>[2x]VEYRNWSKPQCQITGFAPFSKDNSIRLSAGGDIWVTREPYVSCDPV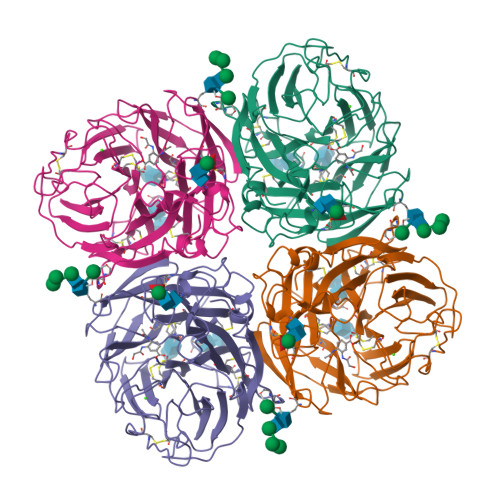KCYQFALGQGTTLDNKHSNDTVHDRIPHRTLLMNELGVPFHLGTRQVCIAWSSSSCHDGKAWLHVCITGDDKNATASFIYDGRLVDSIGSWSQNILRTQESECVCINGTCTVVMTDGSASGRADTRILFIEEGKIVHISPLAGSAQHVEECSCYPRYPGVRCICRDNWKGSNRPVVDINMEDYSIDSSYVCSGLVGDTPRNDDRSSNSNCRDPNNERGTQGVKGWAFDNGNDLWMGRTISKDLRSGYETFKVIGGWSTPNSKSQINRQVIVDSDNRSGYSGIFSVEGKSCINRCFYVELIRGRKQETRVWWTSNSIVVFCGTSGTYGTGSWPDGANINFMPI> MATLKAQHLAKSYKGRQVVRDVSMSIDSGQIVGLLGPNGAGKTTCFYMIVGLVQADQGVVRIDEQNVTHLPMHGRARAGIGYLPQEASIFRKLSVSDNIMAILETRSDLDRNGRKEALEGLLQEFHIHHIRDNLGMSLSGGERRRVEIARALASAPKFILLDEPFAGVDPISVGDIKQIIHHLKAKGIG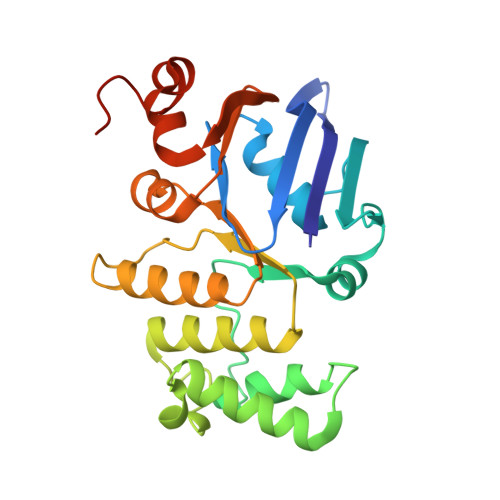ILITDHNVRETLDICETAYIVNDGQLIAEGDAESILANDLVKEVYLGHEFRLHHHHHH> XAAALAAALAQA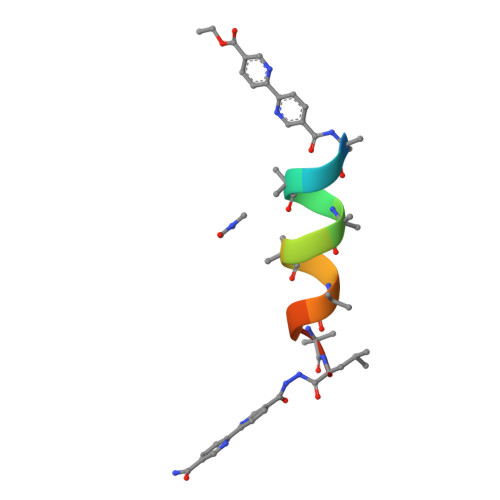LX> MEGEMQRHIKLTKAQTTPVVLVVGDPGRVDKVKVLCDSYVDLAYNREYKSVECTYKGQKFLCVSHGVGSAGCAICFEELMNNGAKVIIRAGSCGSLQPTQMKRGDICICNAAVREDRVSHLMIYSDFPAVADYEVYATLNQVAEELKVPVFNGISLSSDMYYPHKIIPTRLEDYSKANVAVVEMEVATLMVMGTLRKVKTGGIFIVDGCPLKWDEGDFDNNLVPERLENMIKISLETCARLAKKYLEHHHHHH

Purine nucleoside phosphorylase (PNP) is central to purine salvage mechanisms in Plasmodium parasites, the causative agents of malaria. Purine nucleoside phosphorylase (PNP) in Plasmodium forms a key enzyme in the recycling of predominantly host-derived purines, catalysing the phosphorolysis of inosine to produce the major purine precursor for the salvage pathway, hypoxanthine, and ribose-1-phosphate. Crystal structures and sequence homology studies have distinguished two broad families of PNP enzymes: those that form trimers (such as the mammalian PNPs, Type 2) and those that are hexameric (such as E.coli PNP (EcPNP), Type 1). Crystallographic studies of PfPNP have shown it forms a hexameric assembly suggesting its closer alignment with the Type 1 PNP group, although functionally it has been noted that, unlike other hexameric PNPs, adenosine is not a substrate for PfPNP.

The PvPNP crystal structure was refined against 1.85 Å resolution data and the model contains all of the protein residues with the exception of the disordered active site loop (residues 212–224). The crystallographic asymmetric unit contains a monomer of PvPNP which adopts the familiar single-domain fold topology described previously for hexameric PNPs from other species. The nucleoside binding site of the PvPNP enzyme in this structure is observed to be empty although there is electron density consistent with three bound water molecules within the substrate binding site. Additionally, an anion – presumably sulphate from the crystallisation buffer which contained 0.2 M LiSO4 – was identified and this anion occupies the phosphate binding pocket of the enzyme. When the R32 symmetry operators are applied, PvPNP is seen to form a hexameric assembly that matches the arrangements previously reported in crystal structures of PfPNP and EcPNP. Presumed to be the biologically-relevant structure, this hexamer is a disc-shaped single-layer with an overall diameter of about 100 Å and a thickness corresponding to the width of a monomer (approximately 50 Å) with an empty central channel of diameter 20 Å. The hexameric PvPNP appears to be assembled from a trimer of dimers, where the dimer pairs are related by a crystallographic three-fold symmetry axis running through the central channel, corresponding to the view in Figure 2. In common with PfPNP, the phosphate/sulphate binding site of PvPNP is formed mainly by two arginine residues (Arg 89 and Arg 46' from the neighbouring monomer), a backbone interaction with Gly 24, and both backbone and side chain interactions with Ser 91. Another arginine, residue 27, also lies in this region, but points away from the bound sulphate in the PvPNP structure. The composition and structure of the base binding pocket in PvPNP is essentially identical to that described for PfPNP, whereas there are substantial differences when compared to this region in the PkPNP structure.1-deoxy-1-(methylamino)-D-allitol | C7 H17 N O5 | 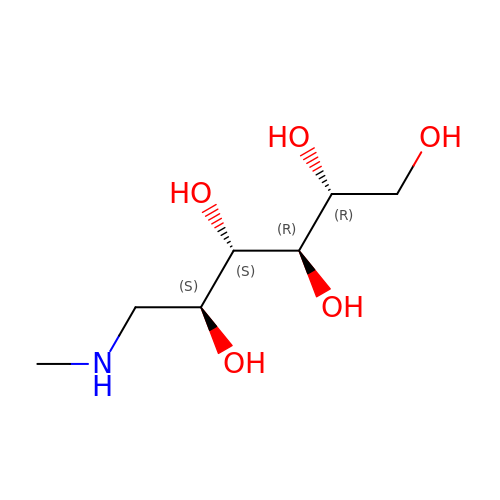MBBZMMPHUWSWHV-BNHYGAARSA-N The human KCTD family contains 25 soluble proteins that share a conserved potassium (K+) Channel Tetramerization Domain (a subtype of ‘BTB domain’) at their N-termini and have variable C-termini. The BTB fold of the Kv and KCTD families has a roughly pyramidal wedge shape and consists of five α-helices and a single β-sheet made from three β-strands. Here, we present novel X-ray crystal structures of the BTB domains of a further five members of the KCTD family and examine the stoichiometry and stability of their multimeric assemblies in solution. Overall, the pyramidal wedge shape of the KCTD family BTB domain creates a versatile scaffold compatible with a range of oligomeric assemblies and geometries that may impact function.

In contrast with the previous work, the expected closed pentameric structure is observed only in KCTD17, whereas the variant C-shaped pentamer, found in one crystal form of KCTD1, is also observed here in KCTD16. The angles between monomers in their assemblies vary from 90° for Kv4.3 to ∼65° for KCTD16, giving rise to observed oligomerization geometries that range from compact to splayed. Evolutionarily distant from these family members are KCTD16 and KCTD1, which belong to closely related clades F and A, respectively. Neither protein binds to Cul3 and both have now been observed to form unusual C-shaped pentamers by X-ray crystallography. We show here that this geometry is also maintained for the KCTD16 BTB in solution. Modest deviations at high q for KCTD16 may be attributed to flexibility and solvation effects not accounted for in the calculated scattering. Binding was observed for each of the BTB domains with the exception of KCTD16, which showed no evidence of Cul3 interaction. In contrast, KCTD16 again demonstrated no interaction with Cul3.

>[15x]SMGSAVPNSFPEVVELNVGGQVYFTRHSTLISIPHSLLWKMFSPKRDTANDLAKDSKGRFFIDRDGFLFRYILDYLRDRQVVLPDHFPEKGRLKREAEYFQLPDLVKLLTPDEIKQSPDE> SNAPDDDAVAIVGAAGRFPGADDLDTFWQQLRAGEDLIADYPGDRFDGGPYAEVVARADFPKFAGRIEGVDRFDADFFHLSRLEAELMDPQHRLALETVWAALENGGYAPARLPENTGVYFGVSGSDYHHLLNASGVAPDGFTATGNAHSMLANRISYVLDVHGPSEPVDTACSSSLVALHRAVEHIRSGRCEMAIAGGVNLLLSVDTFAATHMAGMLSPDGRCKTFSAGADGYVRSEGVAAVLLKPLAQAQRDGDAIWGVVRGSAENHGGRAGSLTAPNGKAQAALIQDAMRGIDPDSIGYVEAHGTGTGLGDPVEVNALDSAYRALRTAEGGPPHAARPCALGSVKTNIGHAESAAGLAGVLKVLLAMRHRELPPALHCDRLNPHLPLDGGFEVVRELRRWEPCTDATGRPWPLRAGVSSFGFGGANAHVVLEAPPVPPAPAEPARPTAPQAIVLSARDDDRLRATAGRLRDFLDRARRDGHAPDLADLAFTLQVGREAMERRLGFVVGS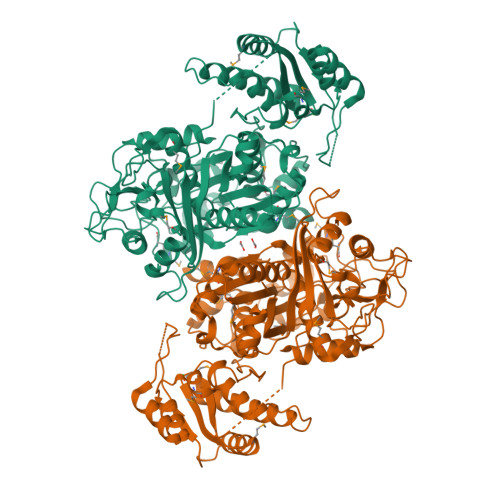MDDVLGTLDRFFAGDEPSGWHTGGIRRSRGAGVRREAEQAPEVTRALHDGRLDRVTALWCDGAPVDWQAMHPTGERRAVRLPAYPFACDRYWVPAVGTAPVPP>[8x]XGEFAQAYKE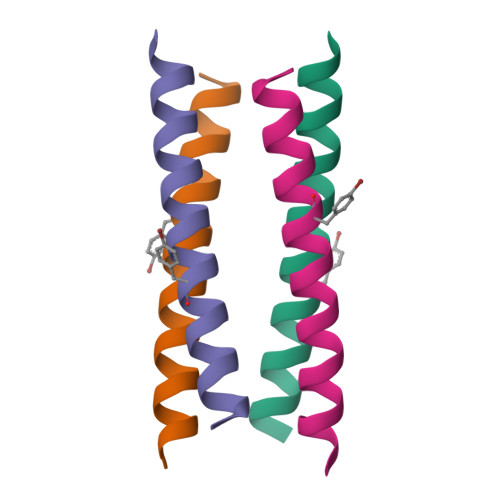FAKAYKEFAYAYKEFAQAYKGX>[2x]GMNN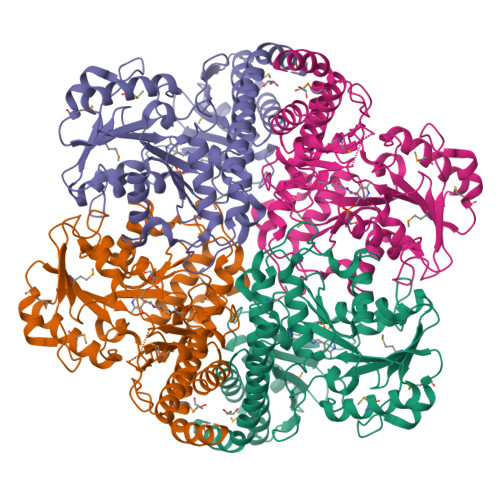IQAIRKKVETQIDDLQNKTDEIAEFNQAKVLDAFQENKVSDFHFHPSTGYGYDDEGRDTLERVYATVFKTEAALVRPQIISGTHAISTVLFGILRPDDELLYITGQPYDTLEEIVGIRKQGQGSLKDFHIGYSSVPLLENGDVDFPRIAKKMTPKTKMIGIQRSRGYADRPSFTIEKIKEMIVFVKNINPEVIVFVDNCYGEFVEYQEPPEVGADIIAGSLIKNPGGGLAKTGGYIAGKEALVDLCGYRLTTPGIGREAGASLYSLLEMYQGFFLAPHVTAQAIKGARFTAAMLAEFGVEADPVWDAPRTDLIQSVSFHNKEKMVAFAQAIQAASPVNAHVLPIGAYMPGYEDDVIMAAGTFIQGASLELTADGPIREPYQLYVQGGLTYEHIKIAVTRAIQKIV> MNDDSQDKIIHDIRIQLRKAATELSRWKLYGSSKWAAEALAGLAEAIDVDQTHSLADESPLRNKQGVPKQMFEIPQNGFGLSETEYDLYLLGSTLFDAKEFDRCVFFLKDVTNPYLKFLKLYSKFLSWDKKSQESMENILTTGKFTDEMYRANKDGDGSGNEDINQSGHQRANLKMVSNEHESQSNISSILKEINTFLESYEIKIDDDEADLGLALLYYLRGVILKQEKNISKAMSSFLKSLSCYSFNWSCWLELMDCLQKVDDALLLNNYLYQNFQFKFSENLGSQRTIEFNIMIKFFKLKVFEELNGQLEDYFEDLEFLLQVFPNFTFLKAYNATISYNNLDYVTAESRFDDIVKQDPYRLNDLETYSNILYVMQKNSKLAYLAQFVSQIDRFRPETCCIIANYYSARQEHEKSIMYFRRALTLDKKTTNAWTLMGHEFVELSNSHAAIECYRRAVDICPRDFKAWFGLGQAYALLDMHLYSLYYFQKACTLKPWDRRIWQVLGECYSKTGNKVEAIKCYKRSIKASQTVDQNTSIYYRLAQLYEELEDLQECKKFMMKCVDVEELLEGIVTDETVKARLWLAIFEIKAGNYQLAYDYAMGVSSGTSQEIEEARMLARE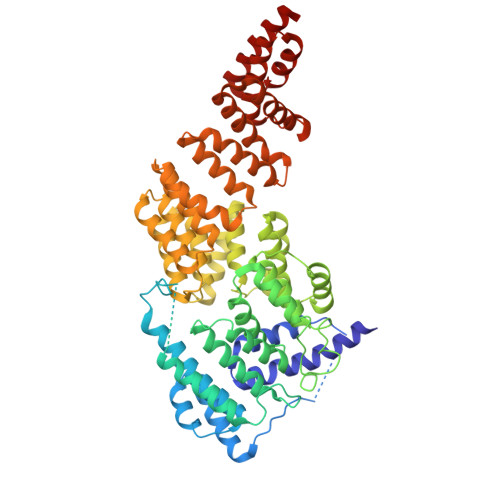CRRHM> MSSTHIEQFMPVKLAQALANSLFPELDSQLRAGRHIGIDDLDNHAFLMDFQEQLEEFYARYNVELIRAPEGFFYLRPRSTTLIPRSVLSELDMMVGKILCYLYLSPERLANQGIFTSQELYEELISLADEGKLMKFVNQRSSGSDLDKQKLQEKVRTTLNRLRRLGMVYFLPNNNNKFTITEAVFRFGADVRSGD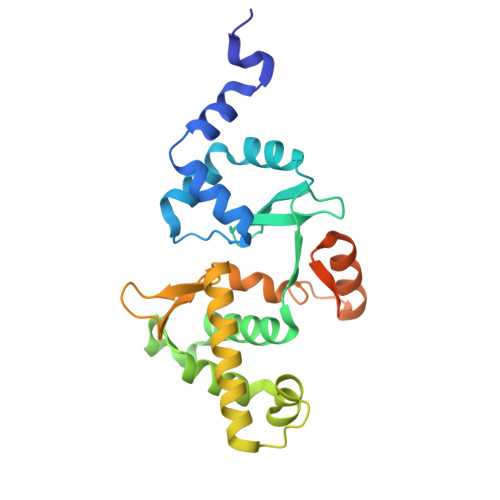DPREIQLRMIRDGEAMPVEGSLSLDDSENDETPDNSAEGAGDEQP> ELTPDQQTLLHFIMDSYNKQRMPQEITNKILKEEFSAEENFLILTEMATNHVQVLVEFTKKLPGFQTLDHEDQIALLKGSAVEAMFLRSAEIFNKKLPSGHSDLLEERIRNSGISDEYITPMFSFYKSIGELKMTQEEYALLTAIVILSPDRQYIKDREAVEKLQEPLLDVLQKLCK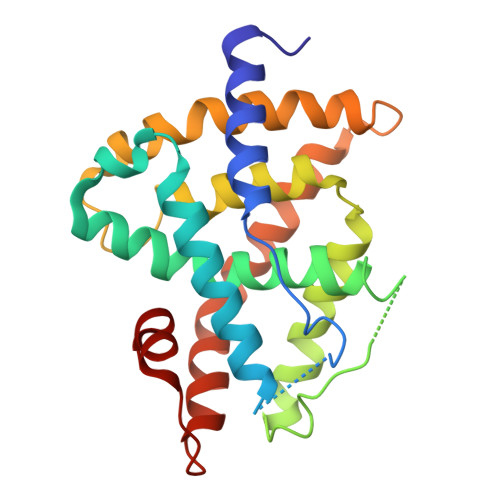IHQPENPQHFACLLGRLTELRTFNHHHAEMLMSWRVNDHKFTPLLCEIWDV>PTPCYISIEGQTQGLITAGACTADSIGDSFVEGHEDEMLVQQFDHVVTVPTDPQSGQPSGQRVHKPFKFTVALNKAVPLLYNALSSGEKLKTVELKWYRTSIEGKQENFFTTKLENASIVDIHCEMPHCQDPAKSDFTQNVTVSLSYRKITWDHVNAGTSGSDDWRKPIE[18x];>[18x]GSLLDEIMAQTRCAPSEEGYDIAKKGVAAFIENLMGSQHSAEPVNKSLVDQMLVELDKKISAQMDEILHNSQFQAMESAWRGLKLFVDRTDFRENNKVEILHVTKDELLEDFEFAPETAQSGLYKHVYSAGYGQFGGEPVGAIIGNYAFTPSTPDMKLLQYMGALGAMAHAPFISSVGPEFFGIDSFEELPNIKDLKSTFESPKYTKWRSLRESEDARYLGLTAPRFLLRVPYDPIENPVKSFNYAENVSASHEHYLWGNTAFAFATRLTDSFAKYRWCPNIIGPQSGGAVEDLPVHVFESMGALQSKIPTEVLITDRKEFELAEEGFIALTMRKGSDNAAFFSANSIQKPKVFPNTKEGKEAETNYKLGTQLPYMMIINRLAHYVKVLQREQIGAWKERQDLERELNSWIKQYVADQENPPADVRSRRPLRAARIEVMDVEGNPGWYQVSLSVRPHFKYMGANFELSLVGRL;>SKEGSVAPKERINIKYIPATGDAQAEVELPLKTLVVGDFKGHA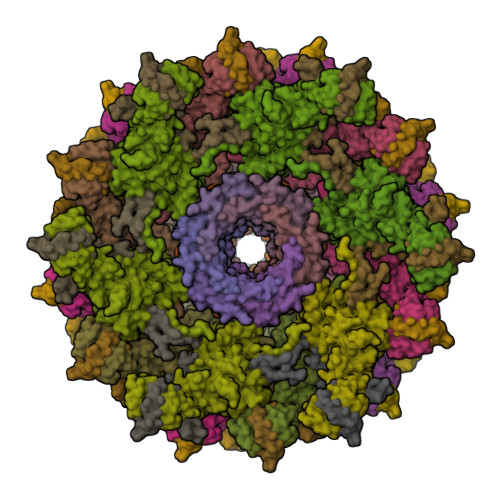EQTPLEERATVTVDKNNFEAVMRESELKITATVKNKLTDDENAELPVELNFKSLADFAPDAVASQVPELKKLIELREALVALKGPLGNIPAFRERLQSLLNSEESREKLLAE[18x]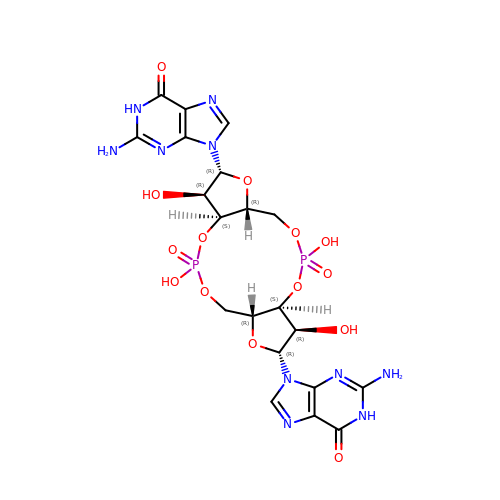9,9'-[(2R,3R,3aS,5S,7aR,9R,10R,10aS,12S,14aR)-3,5,10,12-tetrahydroxy-5,12-dioxidooctahydro-2H,7H-difuro[3,2-d:3',2'-j][1,3,7,9,2,8]tetraoxadiphosphacyclododecine-2,9-diyl]bis(2-amino-1,9-dihydro-6H-purin-6-one) | C20 H24 N10 O14 P2 | PKFDLKSEZWEFGL-MHARETSRSA-N>[2x]KKPLFTKSPRNSASCESTITLQSNLLFTYYKHYFAGIKKVALIGFPDHPNKGDSAIYVAEKKLLDALNIEVVYITAQEADYSASELKSIISDIPRDEFALAFHGGGNFGDLYPDHQHLRELVVRDFPSFTTISFPQSVWYNEQQLLEQASILYAENPNITLVTRDRQSYGFAVDAFGKHNEVLLTPDIVFFMGPIPEIREATPITHDVLILARLDHEGGQQHGAEDYYRDTLNAANLTYSVEDWLLWDPPVAQNPDSSFDDRGQARYEAGAEFLASARVVITDRLHAHILSTLMGIPHIVVENSQMGKITNYHNTWLHGCTLDGVSVVVDSVDKALSLLLEWNEAGYF

The fission yeast pyruvyltransferase Pvg1p, which is localized to the Golgi membrane, attaches pyruvate moieties on oligosaccharides and consequently introduces negative charges on the cell surface. These cell surface negative charges play significant physiological roles, such as intercellular communication. We previously demonstrated that Pvg1p could specifically transfer a pyruvate group onto the α-linked galactose (α-Gal) residues of oligosaccharides. In the Golgi, Pvg1p relies on two transporters, Pet1p and Pet2p, for the supply of its substrate phosphoenolpyruvate (PEP), which is transported from the cytoplasm into the Golgi lumen.

In the present study, in order to elucidate the pyruvyl transfer mechanism of Pvg1p and also to understand the structural basis of its substrate specificity, we first determined the crystal structure of Pvg1p at a resolution of 2.46 Å. The purified Pvg1p was crystallized in the presence of Zn2+. Diffraction analysis of the crystal revealed a structure in which two Pvg1p molecules formed an asymmetric unit with two-fold axis (r.m.s. deviation for the 328 Cα atoms is 0.16 Å). Approximately 928 Å2 of the surface area was buried between the dimer, and it was stabilized by many hydrophobic and hydrogen-bond forming interactions between three α-helices and a β-sheet (α1, α6, α11 and β8). Because the predicted active sites were located far away from the dimer interface, the dimerization of Pvg1p seems to be not essential for the catalysis and substrate binding. The crystal structure of Pvg1p consisted of twelve α-helices and twelve β-sheets, and two α/β/α domains at the N- and C-terminal half regions. The folding pattern of Pvg1p resembled that of the type-B glycosyltransferase, including sialyltransferases. Charged surface representation analysis clearly showed a positively charged cleft situated between the N- and C-terminal halves of Pvg1p, which is suitable for the binding of negatively charged donor substrate PEP. In the proposed model, only the D106 residue is situated within hydrogen bond forming distance of the O6 oxygen of the galactose residue of Lac, whereas both R217 and R337 residues directly interact with PEP. Based on our predicted substrate-binding model of Pvg1p, less pyruvylation was probably due to the steric hindrance posed by the NAc group of the LacNAc-pNP with the H168 of Pvg1p, as a result of which it could not bind properly to the active site of Pvg1p.>[2x]TDILREIGMIARALDSISNIEFKELSLTRGQYLYLVRVCENPGIIQEKIAELIKVDRTTAARAIKRLE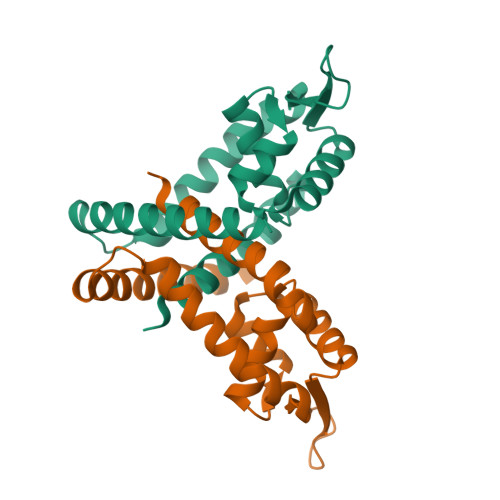EQGFIYRQEDASNKKIKRIYATEKGKNVYPIIVRENQHSNQVALQGLSEVEISQLADYLVRMRKNVSEDWEFVKKG>AGSNKISCLPRVAQNLGYHYSPDLPGFCPIPKELAEHWPVVSNDRYPNCLQITLQQVCELSKPCSAGYMVGQSVFVQTPGVTSYWLTEWVDGKARALPDSLFSSGRFETNSRAFLDEAEEKFAAAHPHACLGEINKSTVGGSAFIFSQYLPPLLPADAVALVGASLAGKAAKAACSVVDVYAPSFEPYLHPETLSRVYKIMIDFKPCRLMV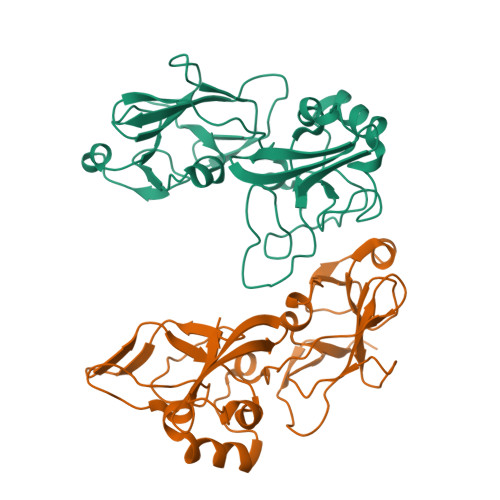WRNATFYVQE[4x]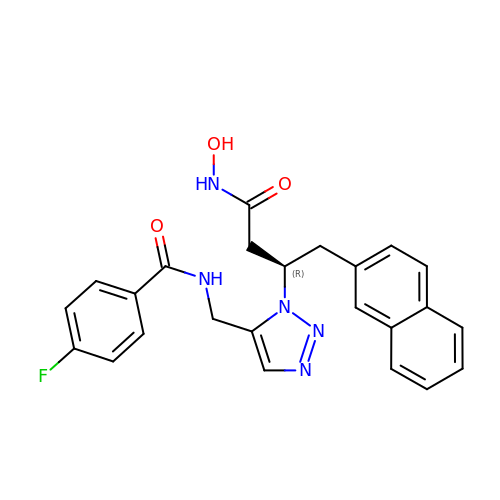4-fluoro-N-({1-[(2R)-4-(hydroxyamino)-1-(naphthalen-2-yl)-4-oxobutan-2-yl]-1H-1,2,3-triazol-5-yl}methyl)benzamide | C24 H22 F N5 O3 | RJVYTCJRTAVEBT-OAQYLSRUSA-N4-[2-(aminomethyl)naphthalen-1-yl]-N-[2-(morpholin-4-yl)ethyl]benzamide | C24 H27 N3 O2 | 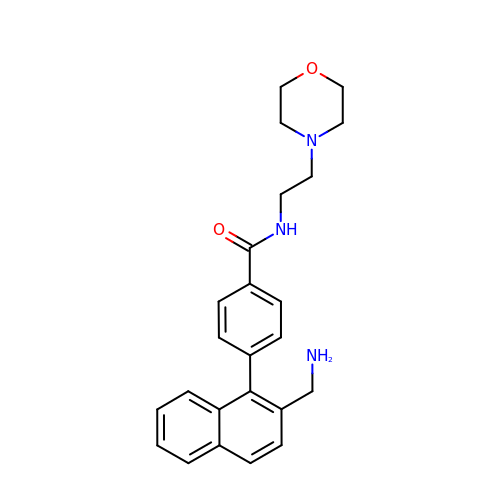LJXMOYXCVXIDDM-UHFFFAOYSA-N> S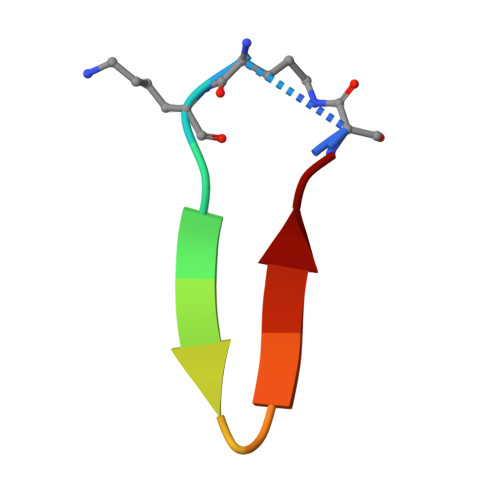AKEYALSGRELT The Zrt-/Irt-like protein (ZIP) family consists of ubiquitously expressed divalent metal transporters critically involved in maintaining systemic and cellular homeostasis of zinc, iron, and manganese. The ZIPs import metal ions, including Zn2+, Fe2+, Mn2+, and other divalent metals in the first row of the d-block region in the periodic table, to cytoplasm. Here, we present a study on a prokaryotic ZIP from Bordetella bronchiseptica (BbZIP) by combining structural biology, evolutionary covariance, computational modeling, and a variety of biochemical assays to tackle the issue of the transport mechanism which has not been established for the ZIP family. The findings, in particular the structure of BbZIP in the apo state and a biochemically validated outward-facing conformation model, consistently support the conclusion that BbZIP is an elevator-type transporter where a four-transmembrane helix (TM) bundle with bound metal substrate slides as a rigid body against the dimeric domain composed of the other static TMs to implement the alternating access mechanism.

While we were trying to crystallize BbZIP in the apo state to reveal alternative conformations, we found that the EDTA-treated protein was prone to form aggregates. During the extensive crystallization trials in lipidic cubic phase, we identified a couple of low pH conditions (~pH 4.0) where diffracting crystals were reproducibly obtained and found to be in the apo state (see below). An unexpected finding is that BbZIP has nine authentic TMs where the extra TM (referred to as α0 hereafter) is located upstream of the eight TMs (α1-α8) conserved in the entire ZIP family. α0 appears to weakly associate with α3 and α6 via smooth surfaces consisting of glycine residues. Inspection of the electron density at the transport site indicated that there was no bound metal, confirming that the protein was crystallized in the apo state. When compared with the metal-bound structure, the binuclear metal center (BMC, the transport sites) underwent large structural changes. Indeed, when Domain II in the apo state structure was aligned with the corresponding region in the cadmium bound structure, a significant displacement of Domain I was revealed. This structural rearrangement is largely attributed to a 9-degree rigid body rotation of Domain I relative to Domain II with the hinge point (of the rotation) located at the extracellular end of α6. In the apo state, the lack of metal ion at the M1 site eliminated a key H177-mediated interaction between α4 and the other TMs in Domain I, leading to the formation of a short 310-helix (spanning residues 176-179) at the bending point of α4. As a result, the cytoplasmic side of α4 underwent a large displacement away from α3 and α7 in Domain II, which likely facilitates the relative movement between the two structurally independent domains.

>[2x]MNQPSSLAADLRGAWHAQAQSHPLITLGLAASAAGVVLLLVAGIVNALTGENRVHVGYAVLGGAAGFAATALGALMALGLRAISARTQDAMLGFAAGMMLAASAFSLILPGLDAAGTIVGPGPAAAAVVALGLGLGVLLMLGLDYFTPHEHERTGHQGPEAARVNRVWLFVLTIILHNLPEGMAIGVSFATGDLRIGLPLTSAIAIQDVPEGLAVALALRAVGLPIGRAVLVAVASGLMEPLGALVGVGISSGFALAYPISMGLAAGAMIFVVSHEVIPETHRNGHETTATVGLMAGFALMMFLDTALG>[4x]SRSAEIMKHGYPGFTNVRTYEDFVLSYDYKTRTAHWVCEHLTPERLKHAEGVDRKLCEFKPDITFPKKFLSQNTDYKCSGFDRGHL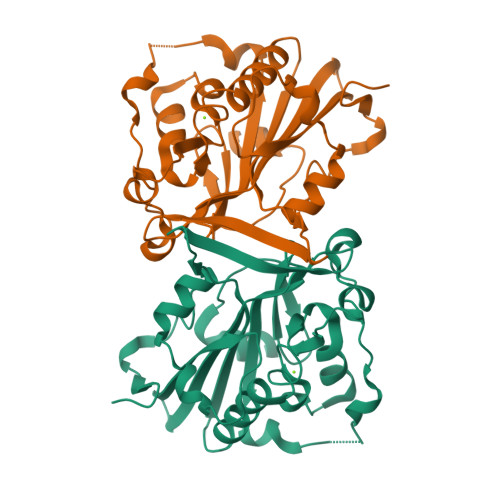AAAGNHRKSQLAVDQTFYLSNMSPQVGRGFNRDKWNDLEMHCRRVAKKMINSYIITGPLYLPKLEGDGKKYIKYQVIGDNNVAVPTHFFKVALFEVTPGKFELESYILPNAVIEDTVEISKFHVPLDAVERSAGLEIFARLDPKSIVKENGAK>[8x]MKETNSEEADSGLAFFRNMYDKYRDAFLSHLNEYSLEEEIKEHISKYYKLLFDYNCLGGKNNRGILVILIYEYVKNRDINSSEWEKAACLAWCIEILQAAFLVADDIMDKGEMRRNKYCWYLLKDVETK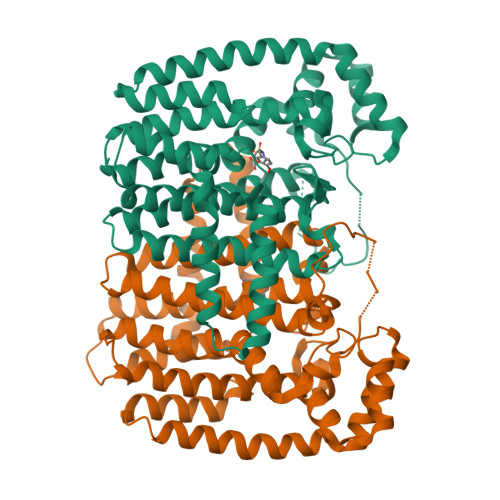NAVNDVLLLYNSIYKLIEIYLRNESCYVDVIATFRDATLKTIIGQHLDTNIFSDKYSDAHREIDVNNINVPEQPVIDINMINFGVYKNIVIHKTAYYSFFLPIVCGMLLAGIAVDNLIYKKIEDISMLMGEYFQIHDDYLDIFGDSTKTGKVGSDIQNNKLTWPLIKTFELCSEPDKIKIVKNYGKNNLACVKVIDSLYEQYKIRKHYESYEKAQKAKILSAINELHHEGIEYVLKYLLEILFTGV Here, inspired by natural and re-engineered protein–peptide systems, we set out to design proteins made out of repeating units that bind peptides with repeating sequences, with a one-to-one correspondence between the repeat units of the protein and those of the peptide. We use geometric hashing to identify protein backbones and peptide-docking arrangements that are compatible with bidentate hydrogen bonds between the side chains of the protein and the peptide backbone. We design repeat proteins to bind to six different tripeptide-repeat sequences in polyproline II conformations. The proteins are hyperstable and bind to four to six tandem repeats of their tripeptide targets with nanomolar to picomolar affinities in vitro and in living cells.

Crystal structures reveal repeating interactions between protein and peptide interactions as designed, including ladders of hydrogen bonds from protein side chains to peptide backbones.

>APEEERIKYVITVVEQIAKDAHRNGQEELAKLAERTAEEAKKATERGEEETLRIVYVIVVVLQIALEAHRNGQEELAKLALRTAEEAIKATERGEEETLRIVYVIVVVLQIALEAHRNGQEELAKLALRTAEEAIKATERGEEETLRIVYVIVVVLQIALEAHRNGQEELAKLALRTAEEAIKATERGEEETLRIVYVIVVVLQIALEAHRNGQEELAKLALRTAEEAIKATERGEEETERIVYDIVVVLQEALEAHRNGEEERAKKALDEARRRIEATERGE[2x];> PLPPLPPLPPLPPLPPLP>MDDKELIEYFKSQMKEDPDMASAVAAIRTLLEFLKRDKGETIQGLRANLTSAIETLCGVDSSVAVSSGGELFLRFISLASLEYSDYSKCKKIMIERGELFLRRISLSRNKIADLCHTFIKDGATILTHAYSRVVLRVLEAAVAAKKRFSVYVTESQPDLSGKKMAKALCHLNVPVTVVLDAAVGYIMEKADLVIVGAEGVVENGGIINKIGTNQMAVCAKAQNKPFYVVAESFKFVRLFPLNQQDVPDKFKYKADTLKVAQTGQDLKEEHP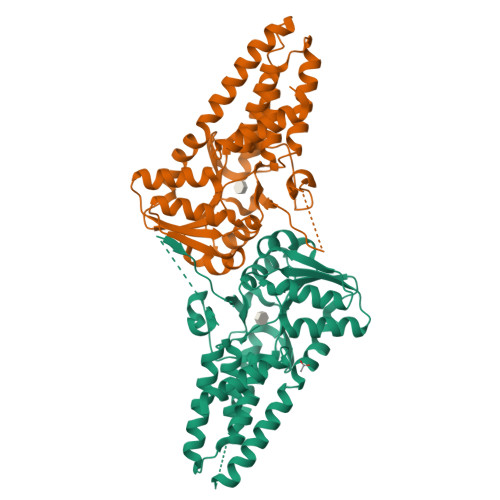WVDYTAPSLITLLFTDLGVLTPSAVSDELIKLYLGGENLYFQ[8x]> MRAEGLGGLERFCSPGKGRGLRALQPFQVGDLLFSCPAYAYVLTVNERGNH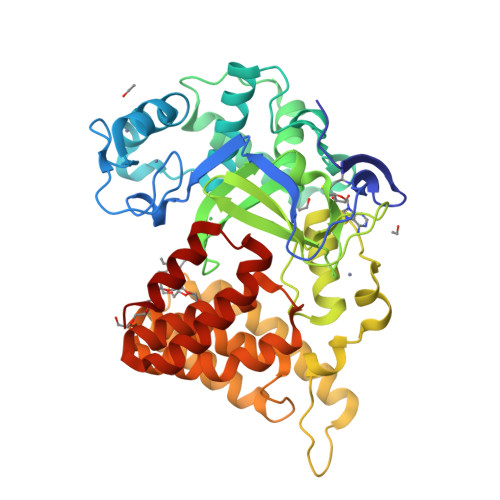CEYCFTRKEGLSKCGRCKQAFYCNVECQKEDWPMHKLECSPMVVFGENWNPSETVRLTARILAKQKIHPERTPSEKLLAVKEFESHLDKLDNEKKDLIQSDIAALHHFYSKHLEFPDNDSLVVLFAQVNCNGFTIEDEELSHLGSAIFPDVALMNHSCCPNVIVTYKGTLAEVRAVQEIKPGEEVFTSYIDLLYPTEDRNDRLRDSYFFTCECQECTTKDKDKAKVEIRKLSDPPKAEAIRDMVRYARNVIEEFRRAKHYKSPSELLEICELSQEKMSSVFEDSNVYMLHMMYQAMGVCLYMQDWEGALQYGQKIIKPYSKHYPLYSLNVASMWLKLGRLYMGLEHKAAGEKALKKAIAIMEVAHGKDHPYISEIKQEIESH> MLSRKGIIPEEYVLTRLAEDPAEPRYRTRERRARFVSKKGNCNVAHKNIREQGRFLQDVFTTLVDLKWPHTLLIFTMSFLCSWLLFAMVWWLIAFAHGDLAPGEGTNVPCVTSIHSFSSAFLFSIEVQVTIGFGGRMVTEECPLAILILIVQNIVGLMINAIMLGCIFMKTAQAHRRAETLIFSKHAVITLRHGRLCFMLRVGDLRKSMIISATIHMQVVRKTTSPEGEVVPLHQVDIPMENGVGGNGIFLVAPL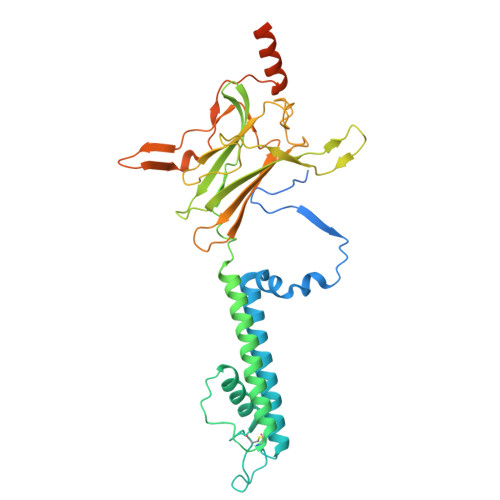IIYHVIDSNSPLYDLAPSDLHHHQDLEIIVILEGVVETTGITTQARTSYLADEILWGQRFVPIVAEEDGRYSVDYSKFGNTIKVPTPLCTARQLDEDRSLLDALTLASSRGPLRKRSVAVAKAKPKFSISPDSLS> MKDSLVLLGRVPAHPDSRCWFLAWNPAGTLLASCGGDRRIRIWGTEGDSWICKSVLSEGHQRTVRKVAWSPCGNYLASASFDATTCIWKKNQDDFECVTTLEGHENEVKSVAWAPSGNLLATCSRDKSVWVWEVDEEDEYECVSVLNSHTQDVKHVVWHPSQELLASASYDDTVKLYREEEDDWVCCATLEGHESTVWSLAFDPSGQRLASCSDDRTVRIWRQYLPGNEQGVACSGSDPSWKCICTLSGFHSR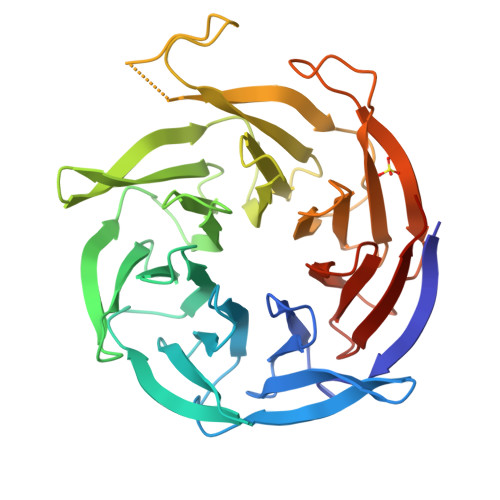TIYDIAWCQLTGALATACGDDAIRVFQEDPNSDPQQPTFSLTAHLHQAHSQDVNCVAWNPKEPGLLASCSDDGEVAFWKYQRPEGLHHHHHH> AINSMSLGASYDAQQANITFRVYSSQATRIVLYLYSAGYGVQESATYTLSPAGSGVWAVTVPVSSIKAAGITGAVYYGYRAWGPNWPYASNWGKGSQAGFVSDVDANGDRFNPN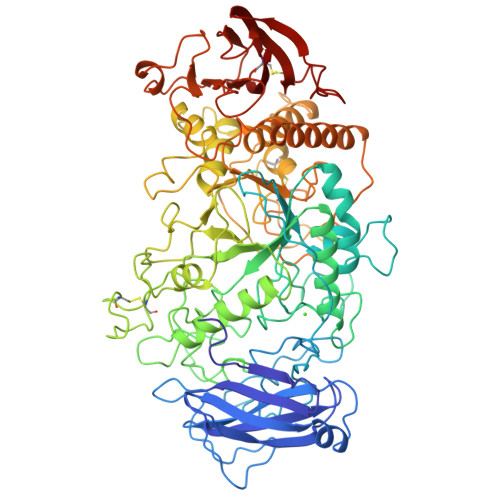KLLLDPYAQEVSQDPLNPSNQNGNVFASGASYRTTDSGIYAPKGVVLVPSTQSTGTKPTRAQKDDVIYEVHVRGFTEQDTSIPAQYRGTYYGAGLKASYLASLGVTAVEFLPVQETQNDANDVVPNSDANQNYWGYMTENYFSPDRRYAYNKAAGGPTAEFQAMVQAFHNAGIKVYMDVVYNHTAEGGTWTSSDPTTATIYSWRGLDNATYYELTSGNQYFYDNTGIGANFNTYNTVAQNLIVDSLAYWANTMGVDGFRFDLASVLGNSCLNGAYTASAPNCPNGGYNFDAADSNVAINRILREFTVRPAAGGSGLDLFAEPWAIGGNSYQLGGFPQGWSEWNGLFRDSLRQAQNELGSMTIYVTQDANDFSGSSNLFQSSGRSPWNSINFIDVHDGMTLKDVYSCNGANNSQAWPYGPSDGGTSTNYSWDQGMSAGTGAAVDQRRAARTGMAFEMLSAGTPLMQGGDEYLRTLQCNNNAYNLDSSANWLTYSWTTDQSNFYTFAQRLIAFRKAHPALRPSSWYSGSQLTWYQPSGAVADSNYWNNTSNYAIAYAINGPSLGDSNSIYVAYNGWSSSVTFTLPAPPSGTQWYRVTDTCDWNDGASTFVAPGSETLIGGAGTTYGQCGQSLLLLISK> MESKVVVPAQGKKITLQNGKLNVPENPIIPYIEGDGIGVDVTPAMLKVVDAAVEKAYKGERKISWMEIYTGEKSTQVYGQDVWLPAETLDLIREYRVAIKGPLTTPVGGGIRSLLVALRQELDLYICLRPVRYYQGTPSPVKHPELTDMVIFRENSEDIYAGIEWKADSADAEKVIKFLREEMGVKKIRFPDHCGIGIKPCSEEGTKRLVRAAIEYAIANDRDSVTLVHKGNIMKFTEGAFKDWGYQLAREEFGGELIDGGPWLKVKNPNTGKEIVIKDVIADAFLQQILLRPAEYDVIACMNLNGDYISDALAAQVGGIGIAPGAN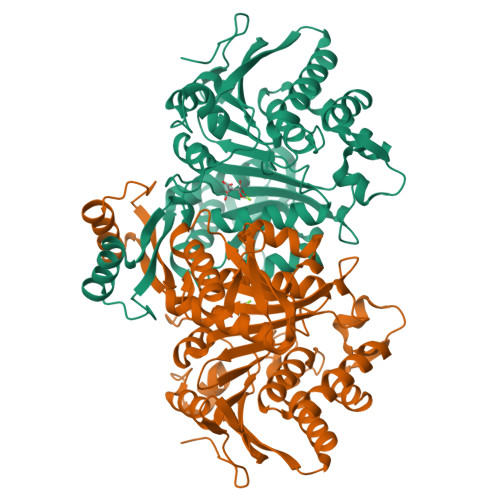IGDECALFEATHGTAPKYAGQDKVNPGSIILSAEMMLRHMGWTEAADLIVKGMEGAINAKTVTYDFERLMDGAKLLKCSEFGDAIIENM> MTIDDSNRLLMDVDQFDFLDDGTAQLSNNKTDEEEQLYKRDPVSGAILVPMTVNDQPIEKNGDKMPLKFKLGPLSYQNMAFITAKDKYKLYPVRIPRLDTSKEFSAYVSGLFEIYRDLGDDRVFNVPTIGVVNSNFAKEHNATVNLAMEAILNELEVFIGRVKDQDGRVNRFYELEESLTVLNCLRTMYFILDGQDVEENRSEFIESLLNWINRSDGEPDEEYIEQVFSVKDSTAGKKVFETQYFWKLLNQLVLRGLLSQ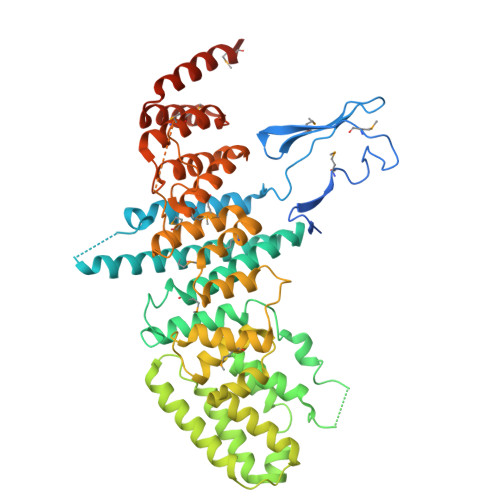AIGCIERSDLLPYLSDTCAVSFDAVSDSIELLKQYPKDSSSTFREWKNLVLKLSQAFGSSATDISGELRDYIEDFLLVIGGNQRKILQYSRTWYESFCGFLLYYIPSLELSAEYLQMSLEANVVDITNDWEQPCVDIISGKIHSILPVMESLDSCTAAFTAMICEAKGLIENIFEGEKNSDDYSNEDNEMLEDLFSYRNGMASYMLNSFAFELCSLGDKELWPVAIGLIALSATGTRSAKKMVIAELLPHYPFVTNDDIEWMLSICVEWRLPEIAKEIYTTLGNQMLSAHNIIESIANFSRAGKYELVKS>GMSDLVFYDVASTGANGFDPDAGYMDFCVKNAESLNLAAVRIFFLNAAKAKAALSRKPERKANPKFGEWQVEVINNHFPGNRNNPIGNNDLTIHRLSGYLARWVLDQYNENDDESQHELIRTTIINPIAESNGVGWDSGPEIYLSFFPGTEMFLETFKFYPLTIGIHRVKQGMMDPQYLKKALRQRYGTLTADKWMSQKVAAIAKSLKDVEQLKWGKGG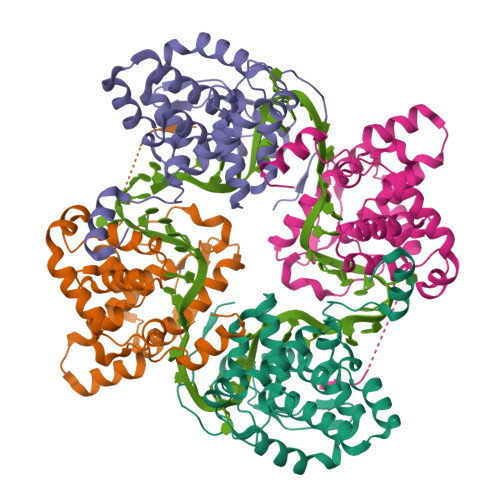LSDTAKTFLQKFGIRLP[4x]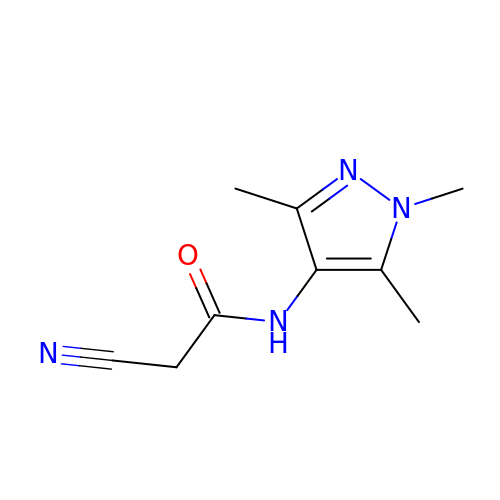2-cyano-~{N}-(1,3,5-trimethylpyrazol-4-yl)ethanamide | C9 H12 N4 O | GCDMTIQQHYQVGI-UHFFFAOYSA-N>LDLFVSPLGRVEGDLDVRVTINDGVVTSAWTEAAMFRGFEIILRGKDPQAGLIVCPRICGICGGSHLYKSAYALDTAWRTHMPPNATLIRNICQACETLQSIPRYFYALFAIDLTNKNYAKSKLYDEAVRRFAPYVGTSYQPGVVLSAKPVEVYAIFGGQWPHSSFMVPGGVMSAPTLSDVTRAIAILEHWNDNWLEKQWLGCSVDRWLENKTWNDVLAWVDENESQYNSDCGFFIRYCLDVGLDKYGQGVGNYLATGTYFEPSLYENPTIEGRNAALIGRSGVFADGRYFEFDQANVTEDVTHSFYEGNRPLHPFEGETIPVNPEDGRRQGKYSWAKSPRYAVPGLGNVPLETGPLARRMAASAPDAETHQDDDPLFADIYNAIGPSVMVRQLARMHEGPKYYKWVRQWLDDLELKESFYTKPVEYAEGKGFGSTEAARGALSDWIVIEDSKIKNYQVVTPTAWNIGPRDASEVLGPIEQALVGSPIVDAEDPVELGHVARSFDSCLVCTVH[2x];>ASVLWFQGGACSGNTMSFLNADEPNVVDLIVDFGLDLLWHPSLGLELGNNAQKVFWDCAKGERPLDIFVFEGTVIEAPNGTGQMDMFAGRPMKDWVTDLAGAAQIVVAIGDCACFGGIPAMEPNPSGSTGLQFHKREKGGFLGPDFRSKMGLPVINVPGCPAHPDWITQILVALATGRAGDITLDDLHRPETFFKTFTQTGCTRVQFFEYKQSTLSFGEGTRTGCLFYEFGCRGPMTHSPCNRILWNRQSSKTRAGMPCLGCTEPEFPHFDLAPGTVFKTQKVSGMIPKEVPEGTDHLTYMGLAAAARIAAPQWSKEDMFVV[2x]

Here we determined the cryo-electron microscopy structure of the Mycobacterium smegmatis hydrogenase Huc and investigated its mechanism. Huc is a highly efficient oxygen-insensitive enzyme that couples oxidation of atmospheric H2 to the hydrogenation of the respiratory electron carrier menaquinone. Huc uses narrow hydrophobic gas channels to selectively bind atmospheric H2 at the expense of O2, and 3 [3Fe–4S] clusters modulate the properties of the enzyme so that atmospheric H2 oxidation is energetically feasible. The Huc catalytic subunits form an octameric 833 kDa complex around a membrane-associated stalk, which transports and reduces menaquinone 94 Å from the membrane.

Because of the flexibility exhibited by this complex, we performed 3D reconstruction of the individual Huc lobe from two datasets, obtaining resolutions of 1.52 Å and 1.67 Å. The head group of menaquinone is stabilized by hydrogen bonding between its oxygen groups and the terminal hydroxyl of Tyr301 and the backbone carbonyl of Lys212, as well as π–π interactions with Tyr229 of HucS. In our 1.67 Å reconstruction, Tyr229 adopts a second conformation that clashes with density corresponding to menaquinone, which shields the proximal [3Fe–4S] cluster from the solvent and may mitigate O2 reduction in the absence of menaquinone, which would lead to the formation of reactive oxygen species. Density maps and the fourth coordinating residue of the 3 iron–sulfur clusters of HucS indicate they all have a [3Fe–4S] configuration. Although the narrow hydrophobic gas channels greatly kinetically favour H2 diffusion over O2, Fourier transform infrared (FTIR) spectroscopy analysis and the cryo-EM structure indicate that the active site of Huc isolated in ambient air is in an oxidized state with a bridging hydroxide ligand. The FTIR vibrational frequencies are consistent with an electron-deficient Ni-B species.> DRHHHHHHKLQHAPPWTEDCRKSTYPPSGPTYRGPVPWYTINLDLPPYKRWHELMVDKGPMLKIIVNSFKNMVNTFVPSGKVMQMVDQKLPDLLGQFSGPYEEEMKGI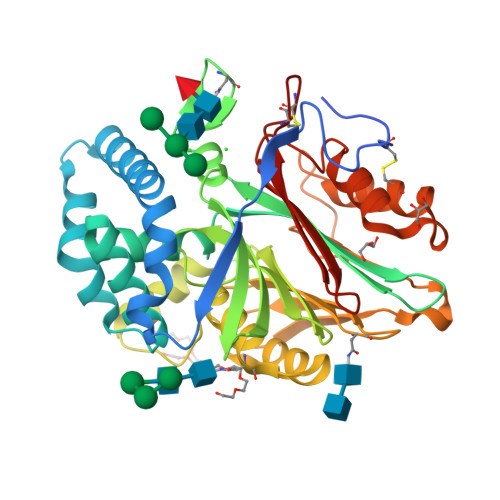ADVTEIPLGEIISFNIFYELFTMATSIITEDKKGHLLHVRNMDFGIFLGWNINNNTWVITEELKPLTVNLDFQRNSKTVFKATSFAGYVGMLTGFKPGQFSLTLNERFSMNGGYLGLLEWILGKKDASWIGFITRSVLENATSYEEAKNILAKTKLLAPAYFILGGNQSGEGCVITRERKDSLDIYELDPKQGRWYVVQTNYDRWKNPLFLDDRRTPAQTCLKRTTQESLSFATLYDILSTKPVLNKLTVFTALMDVTKNHYEAYLRDCPDPCVGW> MELEIRPLFLVPDTNGFIDHLASLARLLESRKYILVVPLIVIN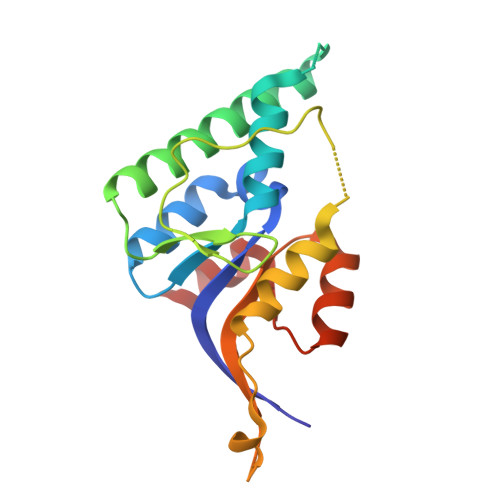CLDGLAKGQETDHRAGGYARVVQEKARKSIEFLEQRFESRDSCLRALTSRGNELESIAFRSEDITGQLGNNDDLILSCCLHYCKDKAKDFMPASKEEPIRLLREVVLLTDDRNLRVKALTRNVPVRDIPAFLTWAQVG>CPPKCRCEKLLFYCDSQGFHSVPNALDKGSLGLSLRHNHITELERDQFASFSQLTWLHLDHNQISTVKEDAFQGLYKLKELILSSNKIFYLPNTTFTQLINLQNLDLSFNQLSSLHPELFYGLRKLQTLHLRSNSLRTIPVRLFWDCRSLEFLDLSTNRLRSLARNGFAGLIKLRELHLEHNQLTKINFAHFLRLSSLHTLFLQWNKISNLTCGMEWTWGTLEKLDLTGNEIKAIDLTVFETMPNLKILLMDNNKLNSLDSKILNSLRSLTTVGLSGNLWECSARICALASWLGSFQGRWEHSILCHSPDHTQGEDILDAVHGFQLCWNLSTTVTVMATTHHHHHH[4x]

Neurexins (Nrxns) are a representative presynaptic organizer family and interact with several different postsynaptic organizers such as neuroligins (NLs), Cbln1–GluD2, and leucine-rich repeat transmembrane neuronal proteins (LRRTMs). LRRTMs are potent postsynaptic organizers that have been shown to instruct presynaptic differentiation. LRRTMs have a leucine-rich repeat (LRR) domain in the N-terminal extracellular domain, which is followed by a single transmembrane domain and a cytoplasmic region. Here, we present the crystal structures of human LRRTM2 LRR domain alone and that in complex with human Nrxn1β LNS domain at 3.15 and 3.4 Å resolutions, respectively.

We consequently obtained diffraction-quality crystals of LRRTM2 (residues 34–371) with the T59L mutation (LRRTM2T59L), which should prevent the attachment of N-glycan at Asn57. One asparagine residue at position 57 is located in close proximity to a crystal contact, which appears to be inhibited by the attachment of N-glycan at Asn57. The interior of the convex face is stabilized by a Phe spine structure, which has also been found in other neuronal LRR proteins such as Nogo receptors, FLRTs, and Slitrks, suggesting their evolutional relationship. The repeat structure at the convex face is partly distorted at LRR7 and LRR8. The convex side of LRR7 forms a short helix and protrudes to LRR8. LRR8 lacks a phenylalanine residue involved in forming the Phe spine. Instead, two phenylalanine residues of the LRR7 convex side are found in the Phe spine by occupying the Phe-spine residue position in LRR8. In these crystals, the C-terminal caps of the adjacent LRRTM2 molecules extensively contact with each other. This contact seems to be stabilized by the intermolecular hydrophobic interaction between Trp333 and His355, which possibly inhibits the co-crystallization of LRRTM2 and Nrxn1β. Therefore, we conclude that the intermolecular contact found in the crystal of apo-LRRTM2T59L is not physiologically important.>HMEMDKRMKSLAMTAFFGELSTLDIMALIMSIFKRHPNNTIFSVDKDGQFMIDFEYDNYKASQYLDLTLTPISGDECKTHASSIAEQLASVDIIKEDISEYIKTTPRLKRFIKKYRNRSDTRISRDTEKLKI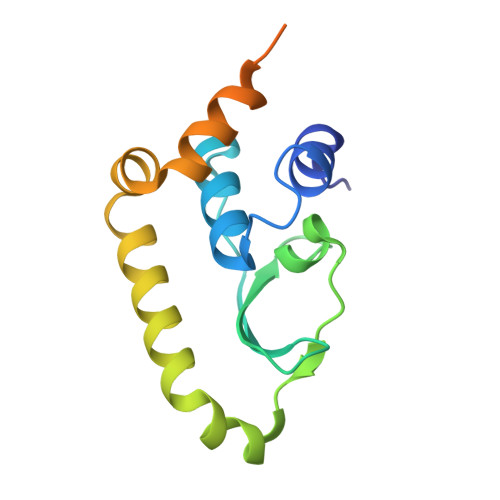ALAKGIDYEYIKDAC[4x]> HHHH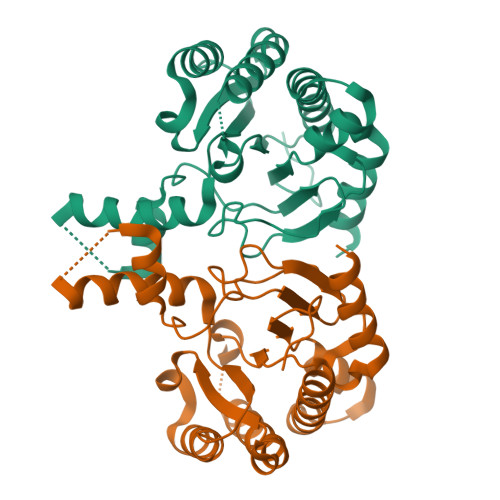HHMFHRAVAPATVPAQTPPAPHTASEGMTSMQHARTAGATGREPPPPLLPPPPLLPPPLPAGTTPAPDRAPGGAHPGNPRHVGVILDGNRRWAEGHGTTLEAAYARGAARVADLVSWCETEGIAVVTVWALSRDNLRRDAAAVGRILDATAVGLAGIAASGRWHIRLIGETDLLPAAPARRLRSVADRTATGSPGTLNVAVAYDGRADIAGAVRGLLRSGVTGGTAAAVRESDVERYLSTAGLPDVDLVIRTSGERRLSGFLPWQTAYAELHFTAALWPAFSFDDFTVALRSYRARRRRFGF> MGWEELTVELEKDGEGLGF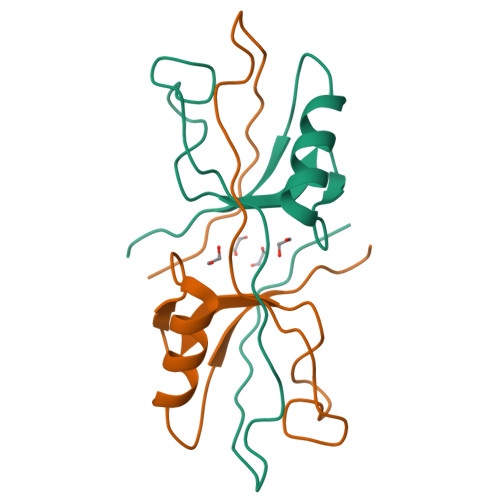SLGDGGIFVSSVVPGGPAARAGRLRVGDRILEVNGVSVEGLTLEEAVKLLRSSGTTVTLTVLRERGGGHHHHHH> MGIYSFWIFDRHCNCIFDREWTLASNSASKQNEEDAKLLYGMIFSLRSITQKLSKGSVKNDIRSISTGKYRV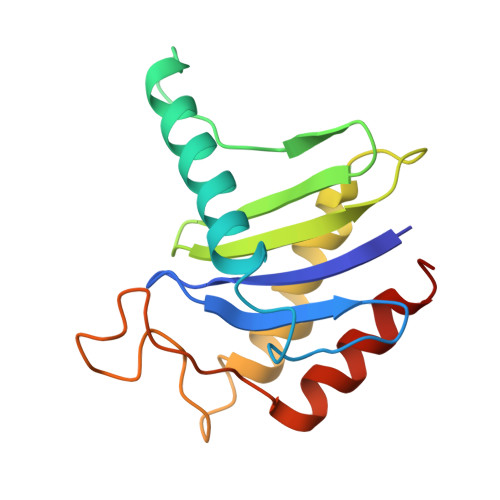HTYCTASGLWFVLLSDFKQQSYTQVLQYIYSHIYVKYVSNNLLSPYDFAENENEMRGQGTRKITNRNFISVLESFLAPMVNQ> MEDTAVETKAKPEKYGSFSEDSLYSLLVAELAGQRNRFDIALSNYVVQAQKTRDP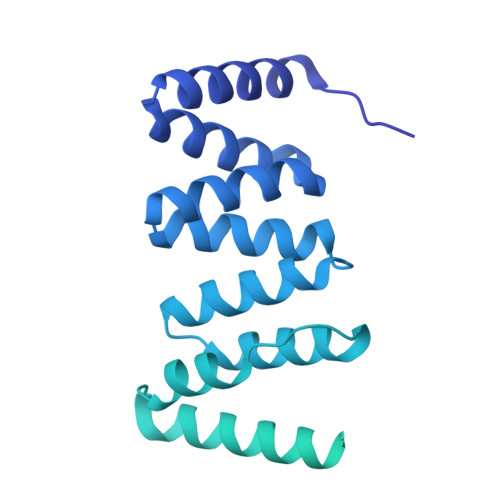GVSERAFRIAEYLGADQEALDTSLLWARSAPDNLDAQRAAAIQLARAGRYEESMVYMEKVLNGQGDTHFDFLALSAAETDPDTRAGLLQSFDHLLKKYPNNGQLLFGKALLLQQDGRPDEALTLLEDNSASRHEVAPLLLRSRLLQSMKRSDEALPLLKAGIKEHPDDKRVRLAYARLLVEQNRLDDAKAEFAGLVQQFPDDDDLRFSLALVCLEAQAWDEARIYLEELVERDSHVDAAHFNLGRLAEEQKDTARALDEYAQVGPGNDFLPAQLRQTDVLLKAGRVDEAAQRLDKARSEQPDYAIQLYLIEAEALSNNDQQEKAWQAIQEGLKQYPEDLNLLYTRSMLAEKRNDLAQMEKDLRFVIAREPDNAMALNALGYTLADRTTRYGEARELILKAHKLNPDDPAILDSMGWINYRQGKLADAERYLRQALQRYPDHEVAAHLGEVLWAQGRQGDARAIWREYLDKQPDSDVLRRTIKRLTGAETP>[8x]MNDNVAWFKQAKYGMMIHWGLYSLLAGEYRGESSSAYAEWIQSKFQIPNAEYGNLATAFNPLYFDAKKIVALAKQCGMQYLVVTTKHHDGFAMYHSKVDAYNVYDATPFHRDIIGELAEACQKAGLKFGLYYSQDLDWHDPNGGGYKSNDVETAGTTWDNSWDFPDEDQKNFDLCFDNKILPQIKEIMSNYGDIATAWFDVPMTLSEAQSQTIYDTVRELQPNCLINSRLGNGKYDFVSLGDAEIPKNKEDMNKTDVDYNEITGFKPSPLGLYETAGTINDSWGFSYHDQNWKTPRTLYRYKQHLNDFGINYLLNVGLDPLGRVPMMAEENLLAAKALEDEANRL

Lactobacillus casei produces a GH29A α-fucosidase, AlfC, that is ~104-fold more active on α(1-6)-fucosyl linkages compared to other linkages. This enzyme is particularly relevant because α(1-6) linkages form the basis of human core fucosylation, which significantly impacts the function of glycoproteins such as antibodies. AlfC is a single-domain enzyme that adopts a (β/α)8 fold typical of GH29 enzymes, with an active site at the center of the barrel. Our results suggest that AlfC employs a conserved hydrolytic mechanism with a specific subsite that accommodates GlcNAc in α(1,6)-linkages, while AlfC tranfucosidase mutants work by shifting equilibrium between open and closed conformations of an active-site loop.

In contrast, N243A showed very high activity (~90% yield with respect to the acceptor GlcNAc), equal to or exceeding the yield of E274A. E39A produced very low yields (~5%), while N243A again equaled the yields (~80%) provided by E274A. We solved the X-ray crystal structures of both of these enzymes. They exhibited no major conformational changes compared to AlfCWT, with CαRMSD < 0.25 Å for each of the enzymes. AlfCN243A was nearly identical to wild-type, including at the site of mutation. This is not surprising, as N243 does not form contacts with any other residues in the AlfC crystal structures. The differences in dynamics for AlfCN243A were more subtle, with this enzyme displaying increases in deuteration in some regions, and decreases in others, both less pronounced than in AlfCE274A. However, like in AlfCE274A, the region containing D242 showed increases in deuteration, suggesting that this enzyme might also sample more open conformations. There was also a large (103-fold) decrease in turnover for N243A, implicating a role for this residue in catalysis. Furthermore, in our studies of AlfCN243A presented here, we showed that the fucose that gets added can be hydrolyzed by AlfCWT following treatment with EndoS2.To gain more information regarding the dynamics of the OMF tunnelling mechanism, we focused our interest on OprN, the OMF protein associated with the MexEF complex within P. aeruginosa. This efflux pump is implicated in the resistance to fluoroquinolones, the most used antibiotic class. As a representative member of the OMF family, OprN structure shows two main domains: a channel of 100 Å long located in the periplasm, also known as the α-domain, and a β-barrel of 30 Å long inserted in the outer membrane. The protein channel is closed by a lid of three β-turns at the extracellular side and occluded by a constriction of three a-coiled-coils at the periplasmic side, which gating mechanism is probably ruled by an iris-like movement.

The OprN channel of the drug transporter MexEF-OprN was analysed in the presence of xenon by X-ray diffraction. OprN-wt and OprN-Xe structures perfectly match each other with a Cα rms deviation of 0.21 Å over 1352 atoms of the trimer, suggesting an overall protein fold unaffected by the xenon interaction. According to the anomalous map, 18 peaks were located in OprN-Xe electron density. Among these peaks, 17 were identified as xenon atoms, according to their high hydrophobic environment, and one was attributed to an opportunistic nickel cation coordinated by the His-tag in subunit C. The main feature of the OprN-Xe structure is a site of xenon with 100% occupancy, named M1. This site is located on the non-crystallographic three-fold axis running along the channel at the periplasmic extremity of OprN. The xenon is trapped in sandwich between the three symmetry-related Leu 405 forming a tight hydrophobic constriction of the channel at that extremity. The xenon cavity is lined on the other side by the three symmetry-related Asp 409, part of a key circular salt bridge with Arg 412, two residues also highly conserved in OprM (Asp 416—Arg 419, respectively). In addition to the M and S sites all located in the a-domain, seven additional xenon atoms are observed at the level of the β-barrel domain. Even if xenon cannot be considered as an inhibitor, it is likely to hamper in the specific case of OMF's the two proposed transport mechanisms: the iris-like mechanism on the periplasmic side, by filling this constricted key-cavity along the channel, and the overall concerted stretch/rotation mechanism by filling specific hydrophobic cavities, built by the coiled-coil long helices forming the cylindrical scaffold of the α-domain.

>[3x]CTVGPDYRTPDTAAAKIDATASKPYDRSRFESLWWKQFDDPTLNQLVEQSLSGNRDLRVAFARLRAARALRDDVANDRFPVVTSRASADIGKGQQPGVTEDRVNSERYDLGLDSAWELDLFGRIRRQLESSDALSEAAEADLQQLQVSLIAELVDAYGQLRGAQLREKIALSNLENQKESRQLTEQLRDAGVGAELDVLRADARLAATAASVPQLQAEAERARHRIATLLGQRPEELTVDLSPRDLPAITKALPIGDPGELLRRRPDIRAAERRLAASTADVGVATADLFPRVSLSGFLGFTAGRGSQIGSSAARAWSVGPSISWAAFDLGSVRARLRGAKADADAALASYEQQVLLALEESANAFSDYGKRQERLVSLVRQSEASRAAAQQAAIRYREGTTDFLVLLDAEREQLSAEDAQAQAEVELYRGIVAIYRSLGGGWQPSAHHHHHH>[2x]MEMILEEKDASDWIYR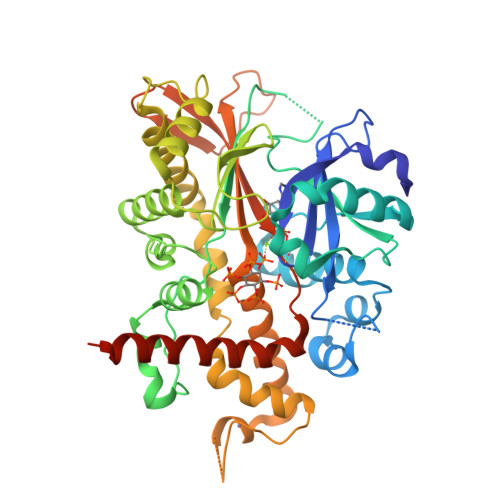GEGGANLVLAYAGSSPLFVGKVIRIQKARRNDKAIKNSNGVVSVLTSDEQHLWRENNELISSPNKEVLEQRYVQNVIIPLLGPKHVDAGVRVSVSKEFLECVDKKVTKQRPLWRVNAANVDTSHDSALILNDHSLFSQGITSGGDCISVEIKPKCGFLPTSRFIGKENMLKTSVSRFKMHQLLKLEYIEISEESEYDPLDLFSGSKERVLEAIKALYSTPQNNFRVFLNGSLILGGSGESTGRTSPEIGYAFEDALKGFIQSEDGHRTECFLQLVSDAVYGSGVLDRLLEIQKLDKLDIEGAIHCYYDIINQPCPICKEGRPLEAELSLHALPLDESLKIVKEYLIAATAKDCSIMISFQSRNAWDSEPSGDYVSLKPTNQTFDYKVHFIDLSLKPLKRMESYYKLDKKIISFYNRKQKAENTAEQIGNSKPSHS>[6x]MLPRPSGTYAGLPIADYGDAPPLSTKTMFWRTSPEKLPPGAWEPAYLGSKDERVDGPSLQQVMRDQLKPYSEPRGLLPPQEILDAVCDAIENRLENTLEPQKPWTFKKACESLDKNTSSGYPYHKQKSKDWTGSAFIGDLGDQATHANNMYEMGKSMRPIYTAALKDELVKPDKIYGKIKKRLLWGSDLGTMIRAARAFGPFCDA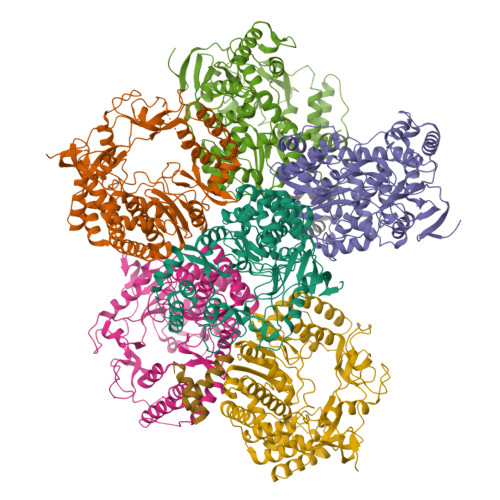LKETCIFNPIRVGMSMNEDGPFIFARHANFRYHMDADYTRWDSTQQRAILKRAGDIMVRLSPEPDLARVVMDDLLAPSLLDVGDYKIVVEEGLPSGCPCTTQLNSLAHWILTLCAMVEVTRVDPDIVMQESEFSFYGDDEVVSTNLELDMVKYTMALRRYGLLPTRADKEEGPLERRQTLQGISFLRRAIVGDQFGWYGRLDRASIDRQLLWTKGPNHQNPFETLPGHAQRPSQLMALLGEAAMHGEKYYRTVASRVSKEAAQSGIEMVVPRHRSVLRWVRFGTMDAETPQERSAVFVNEDAAALEHHHHHH>[4x]SMESLAPFGYNKVSFKQTHHHYCGFYSLNILANIIDNVVVVNGKQYPVSDETAIDWAYDGVDTIVCEKRLVYTEREWPLHTPIYNINNQIVGLVTHGVQLSSQEYCYAVQDGFNLYNNHLTGMNLIVREKKKLIAYADREFDNKSELQIYIEETQKKNCNILGYGAILYHVNKKNAQLILHNNGLQISNSRLRKNVFGNI

Poxviruses are large DNA viruses which replicate exclusively in the cytosol, and encode poxvirus immune nucleases (poxins) to degrade 2′3′-cGAMP and prevent STING activation (Eaglesham et al., 2019). While baculovirus and lepidopteran poxin homologs share <25% identity with VACV poxin, they are functional nucleases and retain 2′3′-cGAMP-specific cleavage activity. New poxin structures include the alphabaculovirus Autographa californica nucleopolyhedrovirus (AcNPV) poxin from Group 2, lepidopteran host poxins from the moth Trichoplusia ni and the monarch butterfly Danaus plexippus in Group 3, and the betabaculovirus Pieris rapae granulovirus (PrGV) poxin from Group 4. In spite of dramatic sequence divergence, poxin structures from each group reveal a shared core fold and head-to-tail dimeric architecture confirming poxins as a single enzyme family.

Group four is formed by poxin proteins from the genomes of several additional lepidopteran viruses: betabaculoviruses (also called granuloviruses), cypoviruses (double-stranded RNA viruses in the family Reoviridae), and betaentomopoxviruses (Silva et al., 2020). The new poxin structures trap a post-reaction state following 2′3′-cGAMP cleavage and allow direct comparison with the catalytic mechanism of VACV poxin. Strikingly, despite sharing <21% identity, each poxin structure contorts 2′3′-cGAMP in an identical strained conformation. Unlike the catalytic triad of histidine, tyrosine, and lysine residues essential for VACV and AcNPV poxin cleavage activity, the active sites of T. ni poxin and PrGV poxin are divergent. The T. ni and PrGV poxin enzymes share the conserved active-site histidine but lack a tyrosine residue entirely. Instead, both proteins contain a second histidine residue adjacent to the first, which forms a contact with the 2′ hydroxyl or 3′ phosphate of the cleaved 2′3′-cGAMP molecule. Further, the T. ni poxin protein shows substitution of the VACV lysine for an arginine residue, whereas the lysine is conserved in PrGV poxin.>[2x]SEQDCKYWPNCANPLCAFRHPTMPPCRNGGECKVPGCKFTHLKTPCKFRPCTNRSCPFLHEEGQRG

The essential heterogeneous nuclear ribonuclearprotein, Nab2 (nuclear abundant poly(A) RNA binding protein 2), a conserved polyadenosine RNA-binding Zn finger protein, functions in polyadenylation, surveillance and the generation of export-competent mRNPs. The S. cerevisiae Nab2 protein contains four domains: an N-terminal PWI-like domain that interacts with NPCs followed by a Gln-rich linker; then an Arg-Gly (RGG) domain required for nuclear import; and finally a domain containing seven tandem CCCH Zn fingers that binds polyadenosine-RNA in vitro, contributes to poly(A) tail length control and is also a checkpoint for proper 3′ processing. The Zn finger domain is essential for Nab2 function and for its binding to poly(A) mRNA, albeit only fingers 5–7 are necessary and sufficient for high-affinity polyadenosine-RNA binding. Here we describe the crystal structure of a complex between polyadenosine RNA and Chaetomium thermophilum Nab2 Zn fingers 3–5 that are homologous to S. cerevisiae fingers 5–7.

Thus, the apparent Mr of Zn fingers 3–5 alone was 8.2 kDa (theoretical 7.7 kDa), that of A8 RNA 3.4 kDa (theoretical 2.6 kDa) and that of fingers 3–5 complexed with A8 RNA 10.6 kDa (theoretical 10.2 kDa for a 1:1 complex). This material was used to generate crystals that had P3121 symmetry with two protein:RNA complexes in the asymmetric unit. The final 2.15 Å resolution structural model had an R-factor of 19.5% (Rfree 20.7%) and excellent geometry, with a final MolProbity score of 0.85 (100th percentile). The final model contained two copies of Nab2 Zn fingers 3–5 (chains A and B) with three Zn atoms each, two acetate molecules, four magnesium ions and 25 water molecules. Additionally, three poly(A) RNA chains were unambiguously placed into the electron density, two of which contained four nucleotides (chains C and D) and the third contained two nucleotides (chain E). Each RNA chain bound to two different protein chains, probably as a result of a form of domain swapping induced by the packing of the molecules into a crystalline lattice. Although the three Zn fingers lacked secondary structural elements, they were packed into a single coherent structure that closely resembled that seen with S. cerevisiae fingers 5–7 (15), albeit superimposition of both structures using their terminal Zn fingers indicated that the middle Zn finger (Zn finger 6 in S. cerevisiae and Zn finger 4 in C. thermophilum) had rotated by ∼53° relative to the terminal fingers. Nab2 protein chain A interacted with five nucleotides overall, with Zn fingers 3 and 5 each binding two adenosines and Zn finger 4 interacting with one. In each binding pocket, the purine base stacked against an aromatic side chain with the hydrophobic region of commonly a lysine or arginine residue masking its other face.Perforin-2 (MPEG1) is thought to enable the killing of invading microbes engulfed by macrophages and other phagocytes, forming pores in their membranes. Perforin-2 (PFN2) has recently been identified as a novel and critically important component of innate immunity conserved throughout the animal kingdom and evolutionarily close to the last common ancestor of the MAC and perforin-1 (7, 10). Because of the presence of a canonical MAC-perforin (MACPF) domain, PFN2 has been proposed to form functional pores in bacterial membranes, leading to bacterial death and control of infection. However, unlike MAC components and perforin-1, PFN2 is initially synthesized as a type I transmembrane protein and found associated with the membranes of intracellular vesicles in which its large ectodomain (consisting mainly of the MACPF domain and a unique P2 domain characteristic of PFN2) projects into the lumen.

We determined structures of the P2 domain in isolation by x-ray crystallography in two crystal forms, with two crystallographically distinct copies in space group P21 at 2.05 Å and eight copies in space group P1 at 3.17 Å. The resolution of the peripheral P2 domain is relatively low in the cryo–electron microscopy (cryo-EM) structure, and in particular, an extended β-hairpin region was not well resolved. However, by determining a structure of the P2 domain in isolation by x-ray crystallography (at 2.05 Å resolution), we were able to build an atomic model for the whole complex into the cryo-EM map. Liposomes containing phosphatidylcholine (PC) and phosphatidylethanolamine (PE) showed no sedimentation of the P2 domain. When adding to these base lipids increasing concentrations of phosphatidylserine (PS) from 5 to 30%, the binding efficiency was gradually enhanced. Given that negatively charged lipids such as cardiolipin, Escherichia coli total lipid extracts, and LPS from E. coli and Salmonella enterica are characteristic of major bacterial membrane lipid species, we also tested and confirmed preferential binding of the P2 domain to these lipids. In contrast, the P2 domain showed almost no binding to liposomes containing sphingomyelin, which is a neutrally charged lipid found in animal cell membranes. Truncating the β hairpin (residues Y427-V452) within the P2 domain (P2Δhairpin mutant) abolished its binding to PS, cardiolipin, and E. coli lipids, confirming the role of this region in membrane binding by PFN2. Thus, membrane binding seems to be conferred exclusively by the tip region of the P2 domain β hairpin.

>ETGGCTNVDSPNFNFQANMDDDSCDAKVTNFTFGGVYQECTELSGDVLCQNLEQKNLLTGDFSCPPGYSPVHLLSQTHEEGYSRLECKKKCTLKIFCKTVCEDVFRVAKAEFRAYWCVAAGQVPDNSGLLFGGVFTDKTINPMTNAQSCPAGYIPLNLFESLKVCVSLDYELGFKFSVPFGGFFSCIMGNPLVNSDTAKDVRAPSLKKCPGGFSQHLAVISDGCQVSYCVKAGIFTGGSLLPVRLPPYTKPPLMSQVATNTVIVTNSETARSWIKDPQTNQWKLGEGTKHHHHHH[2x]> MGSSHHHHHHSSGRENLYFQGMLTEVSDTRIAHKKFGLFYPSVSRPSI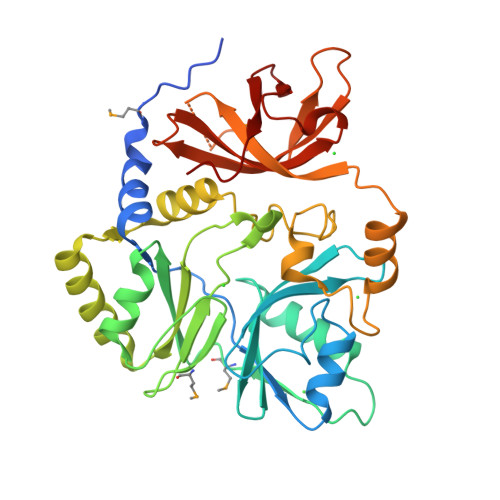FVEGEDRKNFLQGIASQDILKQDEKSLSYSFFLNPKARILFDAWCGNFEDKIALFPPAGTREEFVNHLKKYLFFRTKAKITDMSDHFREIRLVGPETISVLLSLFDNNFSGSSFRMLKNGGYVLIHPTSFQHNLDVGLQADLFIPIDQFETTQKSLEDFTSNKGGVLLDESSYLAYLTEKGIPLFPSELNDSFFPAEAGLDSVGVSYNKGCYVGQEPVTRLKFQGHLNRSLAGFRLEGGPFPKMEFPVTLFNPKDGNEAGILTRTSSSDILGSGIGLGYIKRNFSENGTELLLPDAQLVRVHSLPFV>[3x]GAVETLQGKAATGELLEKSVNTIRFLAIDAVEKANSGHPGLP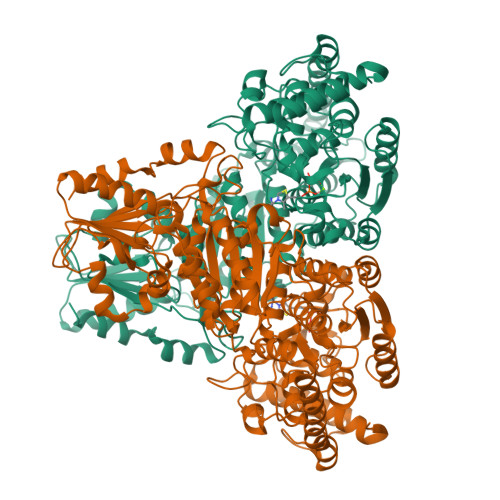MGCAPMGHVLYDEVMRYNPKNPYWFNRDRFVLSAGHGCMLQYALLHLAGYDSVKEEDLKQFRQWGSRTPGHPENFETPGVEVTTGPLGQGIANAVGLALAEKHLAARFNKPDSEIVDHYTYVILGDGCQMEGIANEACSLAGHWGLGKLIAFYDDNHISIDGDTEIAFTEDVSTRFEALGWHTIWVKNGNTGYDDIRAAIKEAKAVTDKPTLIKVTTTIGFGSPNKANSYSVHGSALGAKEVEATRQNLGWPYDTFFVPEDVKSHWSRHTPEGAALEADWNAKFAEYEKKYADDAATLKSIITGELPTGWVDALPKYTPESPGDATRNLSQQCLNALANVVPGLIGGSADLASSNMTLLKMFGDFQKDTAEERNVRFGVREHGMGAICNGIALHSPGFVPYCATFFVFTDYMRGAMRISALSEAGVIYVMTHDSIGLGEDGPTHQPIEHLVSFRAMPNILMLRPADGNETAGAYKVAVLNRKRPSILALSRQKLPHLPGTSIEGVEKGGYTISDNSTGNKPDLIVMGTGSELEIAAKAADELRKEGKTVRVVSFVSWELFDEQSDEYKESVLPAAVTARISIEAGSTLGWQKYVGAQGKAIGIDKFGASAPAGTIYKEYGITVESIIAAAKSF>MSGGGVFTDILAAAGRIFEVMVEGHWETVGMLFDSLGKGTMRINRNAYGSMGGGSLRG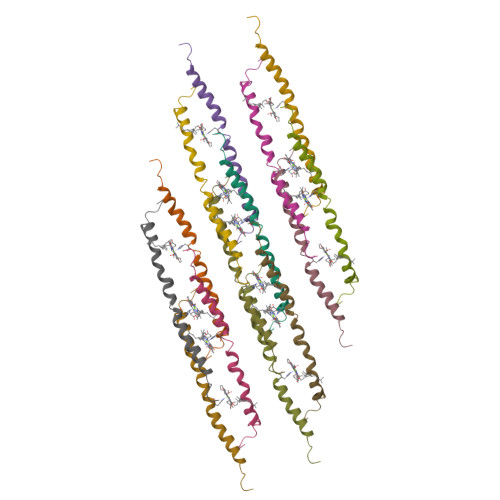S[14x]> GCCCGGAUAGUGUCC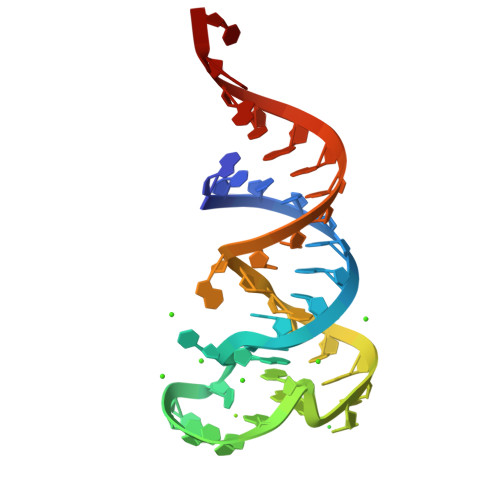UUGGGAAACCGAGUCCGGGCACCA Monkeypox is a disease with pandemic potential. It is caused by the monkeypox virus (MPXV), a double-stranded DNA virus from the Poxviridae family, that replicates in the cytoplasm and must encode for its own RNA processing machinery including the capping machinery. Here, we present crystal structures of its 2′-O-RNA methyltransferase (MTase) VP39 in complex with the pan-MTase inhibitor sinefungin and a series of inhibitors that were discovered based on it. The structure revealed a mixed α/β fold that resembles the Rossmann fold. The catalytic tetrad (Lys41, Asp138, Lys175, Glu218 for MPXV) is absolutely conserved among these unrelated viruses including the conformation of these residues.

We screened a small in-house library of SAH analogs that contains compounds bearing large aromatic or heterocyclic substituents at this position. We identified several compounds that inhibited the VP39 MTase significantly better than sinefungin. Among them, three (TO1111, TO1116, TO1119) had a relatively small substituent (small aliphatic chain or iodine atom) and five (TO427, TO494, TO500, TO504, TO507) had a large aromatic or heterocyclic substituent. Surprisingly, the efficacy of these compounds was very similar (IC50 = 0.08−0.17 µM) and an order of magnitude better than sinefungin (IC50 = 2.3 µM). To confirm our hypothesis that the inhibitors use the discovered water-filled cavity we performed a crystallographic analysis. We used the same approach as with sinefungin and we were able to obtain well diffracting crystals for five compounds (TO427, TO494, TO500, TO507, TO1119). In each case the electron density for the inhibitor was well visible allowing us to unambiguously model the inhibitor although the electron density for the large 7-deaza substituents was less defined than that for the SAH scaffold of the molecule. The crystallographic analysis revealed that in each case the moiety attached to the 7-deaza position is located within the water cavity. However, the inhibitors bearing bulky substituents at this position caused rearrangement of the majority of the water molecules, suggesting that the bulky moieties disrupted the water network within this cavity. TO1119 that only slightly disrupts the water network has IC50 = 128 nM while all the inhibitors with bulky substituents had a lower IC50 except for the only substituent that is able to form a hydrogen bond, the TO500 that possesses a benzimidazole heterocycle. These results suggest that for optimal inhibitor binding it is probably important to disrupt the water network, but it is not important to replace it with other hydrogen bonds.

>MDVVSLDKPFMYFEEIDNELDYEPESANEVAKKLPYQGQLKLLLGELFFLSKLQRHGILDGATVVYIGSAPGTHIRYLRDHFYNLGVIIKWMLIDGRHHDPILNGLRDVTLVTRFVDEEYLRSIKKQLHPSKIILISDVRSKRGGNEPSTADLLSNYALQNVMISILNPVASSLKWRCPFPDQWIKDFYIPHGNKMLQPFAPSYSAEMRLLSIYTGENMRLTRVTKSDAVNYEKKMYYLNKIVRNKVVINFDYPNQEYDYFHMYFMLRTVYCNKTFPTTKAKILFLQQSIFRFLNIPTTSTEKVSHE[2x]> XA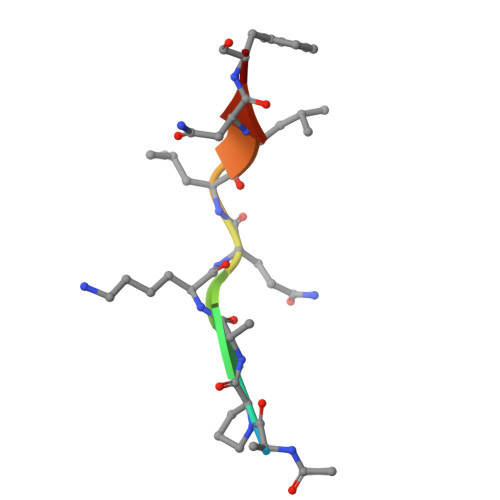PAKQLLNFD>SMEMLTKFESRSSRAKGVAFHPTQPWILTSLHNGRIQLWDYRMGTLL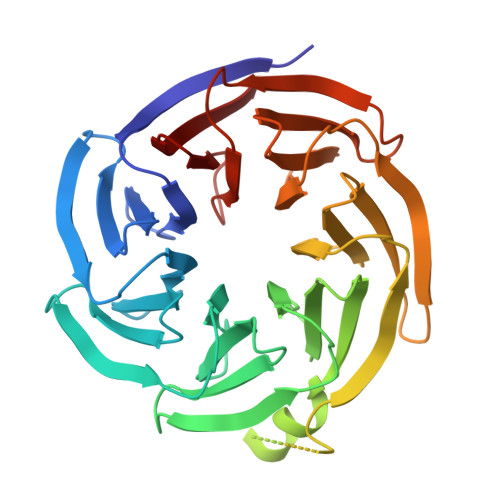DRFDGHDGPVRGIAFHPTQPLFVSGGDDYKVNVWNYKSRKLLFSLCGHMDYVRVCTFHHEYPWILSCSDDQTIRIWNWQSRNCIAILTGHSHYVMCAAFHPSEDLIVSASLDQTVRVWDISGLRMKNAAPVSMSKEDQKAQAHNSKSNDKKGSTDAIVKFVLEGHDRGVNWCAFHPTLPLILSAGDDRLVKLWRMTASKAWEVDTCRGHFNNVSCCLFHPHQELILSASEDKTIRVWDLNRRTAVQTFRRDNDRFWFITVHPKLNLFAAAHDSGVMVFKLE[3x]> MAGDPFVDNGTVSSQRPLRAVPGRYPPGATHLDAAVDTLVRCHAALGRAPSEAEAAVCLLRRLWGRWGNTPVERPGWRSYVAVDGSPFELSAAWNGDGPAEVRVTVEATADPPTPEGNQEAGWEYLRGLSRHPGAATARVLAL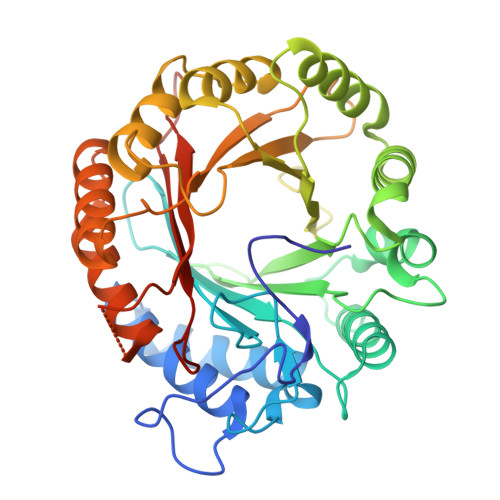EDLFRPQTPHDRCWIMHGMASRPGADPLFKVYLDPDARGAAEAPSVLDEAMDRLGVRAAWQGLRGWLDEHGGSGRIGSLALDLADTDDARVKVYVQHAGLDWADIDRQAAVARGHVPGAFSAALEEITGTEVPPHKPPVTCFAFHRGVGVPTAATLYIPMPAGVPESDARRRSAAFMRRSGLDSAAYLAFLAAATGDGEGVRALQNFVAYRPAAPGGRPRFACYVAPGLYRLEHHHHHH>GPGSMKLCDFEVGLDQPFFLIAGTCVVESEQMTIDTA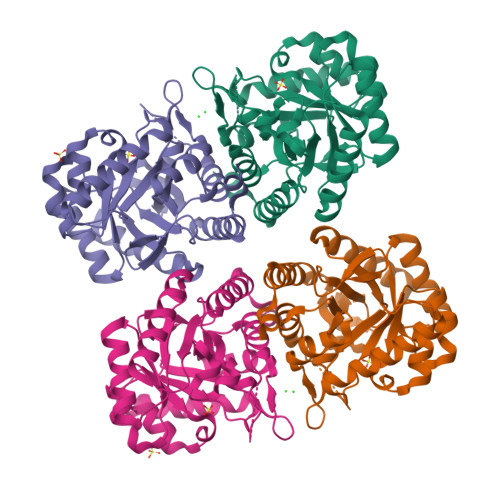GRLKEICEKLNVPFIYKSSYDKANRSSGKSFRGLGMDEGLRILSEVKRQLGLPVLTDVHSIDEIEQVASVVDVLQTPAFLCRQTDFIHACARSGKPVNIKKGQFLAPHDMKNVIDKARDAAREAGLSEDRFMACERGVSFGYNNLVSDMRSLAIMRETNAPVVFDATHSVQLPGGQGTSSGGQREFVPVLARAAVATGVAGLFMETHPNPAEAKSDGPNAVPLNRMGALLETLVTLDQAVKRNPFLENDFN[4x]> CPK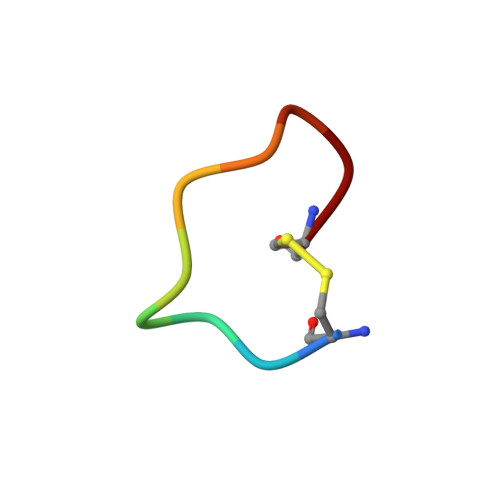RFAALFC SAS-6 organizes the rotationally ninefold symmetric cartwheel, an early assembly intermediate of centrioles that participates in establishing their symmetry and diameter. The cartwheel is organized through the homo-oligomerization of the highly conserved centriolar protein SAS-6. High-resolution crystal structures of zebrafish and C. reinhardtii SAS-6 fragments together with biochemical and biophysical characterizations demonstrated that two dimerization interfaces in SAS-6 mediate this oligomerization: a coiled-coil domain that forms a rod-like parallel dimer; and a globular N-terminal domain that forms a curved head-to-head dimer. SAS-6 is a highly conserved protein that is found in all eukaryotes that have cilia/flagella during some of their life-cycle stages.

However, with the wild-type construct of Lm SAS-697–320, we finally succeeded to find a crystal form of the space-group H3 that diffracted to a resolution of ∼3.5 Å along the l-axis with anisotropy limiting the resolution along the h-k plane to ∼4.2 Å. Using the structure of the Lm SAS-697–274 B–C homo-dimer as a search model, a molecular replacement solution could be found that allowed the subsequent placement of the coiled-coil part present in the construct. The unit cell of the Lm SAS-697–320 crystal form contained three 9-fold symmetric SAS-6 rings with three SAS-6 dimers constituting the ASU. These three dimers were highly similar to each other and overlayed with an rmsd of 0.88 ± 0.29 Å in secondary structure matching with 357 ± 14 selected pairs. The inner diameters of the SAS-6 rings are ∼19 nm and correspond well to the diameters of cartwheel hubs observed in vivo. In the crystal, SAS-6 rings are stacked onto each other. Neighbouring rings interact through inter-digitation of their coiled-coil domains in an antiparallel way. The ASU of the crystal contained six SAS-6 monomers that are labelled from A–F. No clear electron density could be seen for the distal part of the coiled-coil of the A–B dimer, probably due to the lack of stabilizing crystal packing interactions compared to the C–D and E–F dimer. However, we demonstrate that under high protein and precipitant concentrations, a L. major SAS-6 construct crystallized as ninefold symmetric rings with a diameter very similar to cartwheel hubs in vivo; this provides the first unambiguous experimental evidence that SAS-6 is able to form ninefold symmetric cartwheels on its own. However, in our ring structure, both of these critical interfaces are similar in their orientations to those observed in the crystals of the Lm SAS-697–320 F257E and the Lm SAS-697–274 constructs that did not crystallize as rings.

>[6x]GPHMEAVESGVAPPPAVRTARTDLPALASPKHSAEEPQTLLETTVMVSTKMPPHEPQVRPLGVYVRTGRGGPNGVTRVVLVRLTDPTDPFFLFELELLEDDYNAFKQHLELLVDFHGFPRYLVGMLRDIADGASAYELSFVLNSAAVGDSNRGTLRVLETTDFKTVEHISLVLLRQGDAGLKRYLAERFQHYEQSFRASEASRAVITAELQEKIGDLQAANDALRA> SSPGKPPRLVGGPMDASVEEEGVRRALDFAVGEYNKASNDMYHSRALQVVRARKQIPAGVNYFLDVELGRTTCTKTQPNLDNCPFHDQPHLKRKAFCS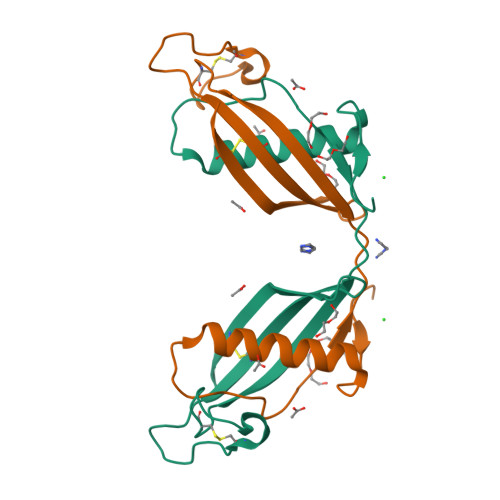FQIYAVPWQGTMTLSKSTCQDA>[60x]MSVEPAGGGGGVKVKAQWIGGTSFSDSVVITSHTRTSMLADRGGYVPVYKQGSHVDSSQPVMGMKTPYSYIDVNALSAHFTPRDFQQLLDEYDEIKPKSLTIAISAIVIKDVATNQTGTTVSDSASGGITVFADDSYDYPYVLGHNQDTLPGHLPGENYVLPQYGYITRGREIDQQNSIVAISDHKTELFFLEHHDAECLGTGDHWSHHYEFPDDLPWRKLSTPNQTLYARHNPIPSSRLAIMTGVDNDGTAIWKRPEGMDVGRLPLNYVPGPALMMPTDTQIRNTTFRDPVAIGNPATSDRYSVAPLVHQPW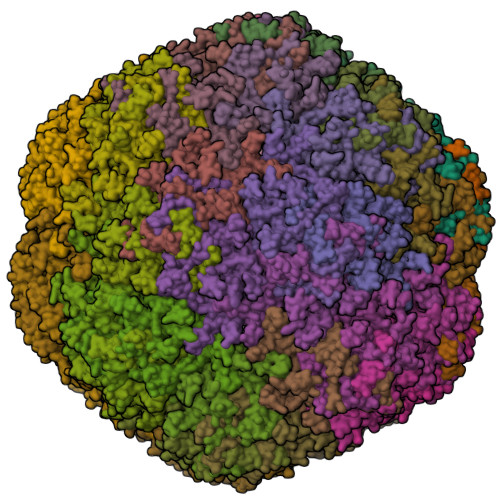SVRTEEWLANKTDYAVHNYLGGVAYTRRKHEESYDKHEEDRDGRVTNPSRVVQIDGDLAAPHVGHTFFVPGHTRVTSGGTDTVYSPKLYQEPVFPLFPGAVWNPNPLSYDCQIWTKIPNTECHFFAQYPLLGGWGVLTPPPMIFVKLRSQPGPPSPGAHTVPQSNLNQYAIFHLHYSMQFLVKRRKRSRRHNPEKPAPFPTTDSGRMPFTLANSLKDPNTPVYEVPSDQWIARNYSHLL> MGSSLRPLYMDVQATTPLDPRVLDAMLPYLINYYGNPHSRTHAYGWESEAAMERARQQVASLIGADPREIIFTSGATESNNIAIKGVARFYRSRKKHLITTQTEHKCVLDSCRSLEAEGFQVTYLPVQKSGIIDLKELEAAIQPDTSLVSVMTVNNEIGVKQPIAEIGRICSSRKVYFHTDAAQAVGKIPLDVNDMKIDLMSISGHKIYGPKGVGAIYIRRRPRVRVEALQSGGGQERGMRSGTVPTPLVVGLGAACEVAQQEMEYDHKRISKLSERLIQNIMKSLPDVVMNGDPKHHYPGCINLSFAYVEGESLLMALKDVALSSGSACTSASLEPSYVLRAIGTDEDLAHSSIRFGIGRFTTEEEVDYTVEKCIQHVKRLREMSPLWEMVQDGIDLKSIKWTQH;> MAASSRAQVLALYRAMLRESKRFSAYNYRTYAVRRIRDAFRENKNVKDPVEIQTLVNKAKRDLGVIRRQVHIGQLYSTDKLIIENRDMPRT;> STIEERVKKIIGEQLGVKQEEVTNNASFVEDLGADSLDTVELV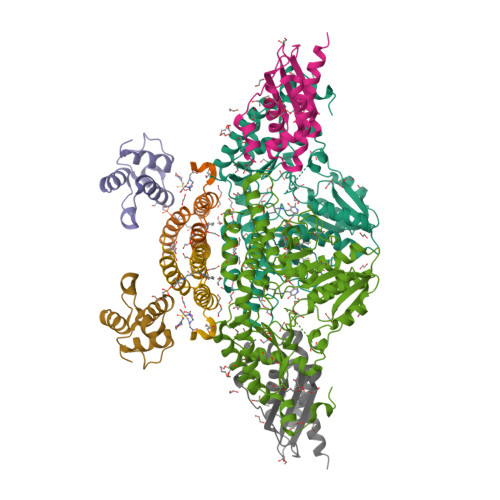MALEEEFDTEIPDEEAEKITTVQAAIDYINGHQA;> MADHKKVVDHYENPRNVGSLDKTSKNVGTGLVGAPACGDVMKLQIQVDEKGKIVDARFKTFGCGSAIASSSLATEWVKGKTVEEALTIKNTDIAKELCLPPVKLHCSMLAEDAIKAALADYKLKQEPKKGEAEKKLEHHHHHH>GMILLIDNYDSFTWNLYQYFCELGADVLVKRNDALTLADIDALKPQKIVISPGPCTPDEAGISLDVIRHYAGRLPILGVCLGHQAMAQAFGGKVVRAAKVMHGKTSPITHNGEGVFRGLANPLTVTRYHSLVVEPDSLPACFDVTAWSETREIMGIRHRQWDLEGVQFHPESILSEQGHQLLANFLHR[2x];>QGHMKTLSPAVITLLWRQDAAEFYFSRLSHLPWAMLLHSGYADHPYSRFDIVVAEPICTLTTFGKETVVSESEKRTTTTDDPLQVLQQVLDRADIRPTHNEDLPFQGGALGLFGYDLGRRFESLPEIAEQDIVLPDMAVGIYDWALIVDHQRHTVSLLSHNDVNARRAWLESQQFSPQEDFTLTSDWQSNMTREQYGEKFRQVQEYLHSGDCYQVNLAQRFHATYSGDEWQAFLQLNQANRAPFSAFLRLEQGAILSLSPERFILCDNSEIQTRPIKGTLPRLPDPQEDSKQAVKLANSAKDRAENLMIVDLMRNDIGRVAVAGSVKVPELFVVEPFPAVHHLVSTITAQLPEQLHASDLLRAAFPGGSITGAPKVRAMEIIDELEPQRRNAWCGSIGYLSFCGNMDTSITIRTLTAINGQIFCSAGGGIVADSQEEAEYQETFDKVNRILKQLEK[2x]

Here, we chose aminodeoxychorismate synthase (ADCS) from Escherichia coli, which consists of a class I glutaminase subunit (PabA) and a synthase subunit (PabB), to investigate the mechanism of glutaminase catalysis regulation and its impact on overall GAT activity. PabB catalyzes the amination of chorismate (Cho) to 4-amino-4-deoxy-chorismate, which is a committed step in folic acid biosynthesis. GATs comprise minimally a glutaminase that produces ammonia, which reacts with a synthase-bound substrate to yield specific nitrogen-containing products. As evidenced by analytical gel filtration and isothermal titration calorimetry (ITC) data, the PabA and PabB subunits form a heterodimeric assembly with a dissociation constant KD = 0.16 ± 0.06 μM.

When Gln was added to the crystallization buffer, we found a glutamyl thioester (Gln-TE) adduct covalently bound to the catalytic aC79 within the glutaminase active site in only one of the two PabA/PabB heterodimers, indicating that under the given crystallization conditions the glutaminase reaction proceeded only to the Gln-TE adduct without performing the final hydrolysis step. This finding is most likely due to structural restraints imposed by the crystal lattice, in line with similar observations in other GAT structures. When Gln forms a covalent adduct with the catalytic aC79, as expected, the glutaminase catalytic triad residue aH168 is in a catalytically competent position, allowing a nucleophilic attack of water on the reactive carbon atom to reconstitute free aC79. In the ADCS structures with Gln-TE bound in the glutaminase active site, we consistently observed a distinct water molecule interacting with active site residues aY127 and aH168. This water molecule is in an appropriate position to hydrolyze the Gln-TE, as illustrated by a close distance of less than 3 Å to the Gln-TE reactive carbon atom, which is subject for nucleophilic acyl substitution, and hence it is referred to as the glutaminase catalytic water molecule. Finally, the reactive carbonyl group of Gln-TE interacts with the main chain amino groups of aG52 and aL80, which together form the oxyanion hole required for glutaminase catalysis by polarization of its carbonyl group. We also found several interactions between the noncatalytic amino group of Gln-TE and residues of both ADCS subunits, including bG207 and bY210 from the PabB subunit, allowing the catalytic center of Gln-TE to be positioned with very high spatial precision, to generate a catalytically competent glutaminase active site arrangement at the PabA/PabB interface. Indeed, we found a rotation by approximately 23° in the principal axis orientation of PabA and PabB subunits induced by the presence of Gln-TE.> MKLILCTVLSLGIAAVCFAAPPKSVIRWCTISSPEEKKCNNLRDLTQQERISLTCVQKATYLDCIKAIANNEADAISLDGGQAFEAGLAPYKLKPIAAEVYEHTEGSTTSYYAVAVVKKGTEFTVNDLQGKTSCHTGLGRSAGWNIPIGTLLHRGAIEWEGIESGSVEQAVAKFFSASCVPGATIEQKLCRQCKGDPKTKCARNAPYSGYSGAFHCLKDGKGDVAFVKHTTVNENAPDQKDEYELLCLDGSRQPVDNYKTCNWARVAAHAVVARDDNKVEDIWSFLSKAQSDFGVDTKSDFHLFGPPGKKDPVLKDLLFKDSAIMLKRVPSLMDSQLYLGFEYYSAIQSMRKDQLTPSPRENRIQWCAVGKDEKSKCDRWSVVSNGDVECTVVDETKDCIIKIMKGEADAVALDGGLVYTAGVCGLVPVMAERYDDESQCSKTDERPASYFAVAVARKDSNVNWNNLKGKKSCHTAVGRTAGWVIPMGLIHNRTGTCNFDEYFSEGCAPGSPPNSRLCQLCQGSGGIPPEKC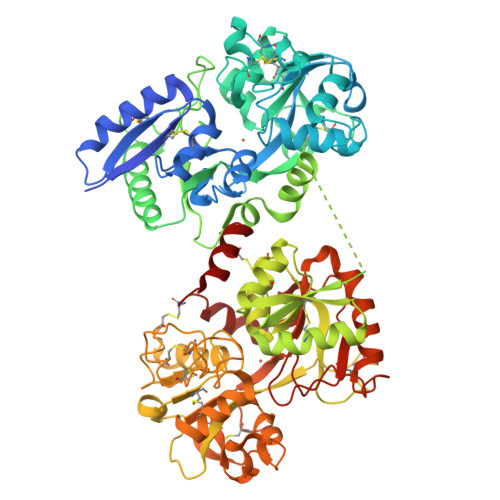VASSHEKYFGYTGALRCLVEKGDVAFIQHSTVEENTGGKNKADWAKNLQMDDFELLCTDGRRANVMDYRECNLAEVPTHAVVVRPEKANKIRDLLERQEKRFGVNGSEKSKFMMFESQNKDLLFKDLTKCLFKVREGTTYKEFLGDKFYTVISSLKTCNPSDILQMCSFLEGK The proteasome of the malaria parasite Plasmodium falciparum (Pf20S) is an advantageous drug target because its inhibition kills P. falciparum in multiple stages of its life cycle and synergizes with artemisinins. The 20S proteasome core particle is composed of two antechambers located between an α-ring and a β-ring and a catalytic chamber centrally located between two β-rings. Unfolded peptide substrates must pass through the antechamber before reaching the catalytic chamber for degradation. We recently developed a macrocyclic peptide, TDI-8304, that is highly selective for Pf20S over human proteasomes and is potent in vitro and in vivo against P. falciparum.

To answer this question, we determined a cryo-EM structure of the partially purified β6A117D mutant Pf20S (Pf20Sβ6A117D) with WLW-vs at 2.58 Å resolution. Because WLW-vs is a β2-specific inhibitor, we were surprised to observe WLW-vs in both β2 and β5 catalytic sites of the Pf20Sβ6A117D. The overall binding mode of WLW-vs in both sites is similar, following an anti-parallel β-strand configuration resembling peptide substrates. In both β2 and β5, the inhibitor is covalently linked to the catalytic Thr-1, the two indole groups at the P1 and P3 sites are inserted into the S1 and S3 pockets, respectively, and the P2 Leu and P4 morpholine face the catalytic chamber. We compared the β6 subunit structures of the wild-type Pf20S and A117D mutant Pf20S, and with the high resolution of the two EM maps, we clearly see that the β6A117D caused a one-residue shift as well as an upside-down flip in the Gly156-to-Ala161 region. In the wild-type β6 structure, Tyr158 points upward to interact with the small hydrophobic Ala117. In the A117D mutant β6 structure, the negatively charged Asp117 has expelled Tyr158 from its wild-type position, causing the observed one-residue shift and the upside-down flip in the Gly156-to-Ala161 region. Furthermore, the flipping of the Gly156-to-Ala161 peptide moves Ser154 away from pyrrolidinone and diminishes the TDI-8304’s affinity for the β5 pocket. Also, the aromatic ring of the Tyr158 at its new position hydrophobically interacts with one indole ring of the WLW-vs. Especially, the hydroxyphenyl ring of Tyr158 interacts with the indole ring of the P3 Trp of the WLW-vs via an offset π-π stacking with a favored vertical distance 3.4 Å, which likely explains why the β2-specific inhibitor WLW-vs also binds in the β5 pocket of the Pf20Sβ6A117D, supporting the observed enhanced inhibition against the β5 activity of the Pf20Sβ6A117D19. By comparing the structures of the Pf20S WT and Pf20S A117D, we unambiguously found that the A117D mutation not only causes a conformational change in the β5 inhibitor binding pockets, but also a substantial conformational change remotely in the β2 active subunit that enhances the binding affinity of a β2 inhibitor.

>[2x]MVRPSQSMYDRHLTIFSPDGNLYQIEYAIKAVKNTNITSVGVKGENCAVIISQKKMATQYISQDKLLDYNNITNIYNITDEIGCSMVGMPGDCLSMVYKARSEASEFLYSNGYNVNAETLCRNICDKIQVYTQHAYMRLHACSGMIIGIDENNKPELFKFDPSGFCAGYRACVIGNKEQESISVLERLLEKRKKKIQQETIDEDIRNTTILAIEALQTILAFDLKASEIEVAIVSTKNRNFTQISEKEIDNYLTYIAERD;>MADGEYSFSLTTFSPTGKLVQIEYALNRVSSSSPALGIRAKNGVIIATEKKSPNELIEENSIFKIQQISEHIGIVYAGMPGDFRVLLKRARKEAIRYSLQYGSEILVKELVKIIASIVQEFTQTGGVRPFGLSLLICGVDVYGYHLYQIDPSGCYFNWMATCVGKDYQNNMSFLEKRYNKDIEIEDAIHTAILTLKESYEGVLNEKNIEIGVAYDNKPFKILTQNEIKDYLIEIE[2x];>[2x]MARRYDSRTTTFSPEGRLYQVEYALEAINNASITIGLITKDGVILGADKVFISKLIDKANNYEKIYKIDKHIFCGVAGLNADANILINQSRLYAQRYLYNYNEVQPVSQLVVQICDIKQSYTQYGGLRPYGVSFLIGGYDTKDGYQLYHTDPSGNYSGWFATAIGTNNLTASSVLKQEWKNDMTLEEGLLLALKTLAKSTDTEIPKSEKIELAYLTNKDGEVYQKYLTEKEIEELIKLYTQKYIKE;>MSYDRAITVFSPDGHLLQVEHALEAVKKGGCAVAIKSSNFAVLAVEKKNIPKLQNPKTTEKLIKLDEHNCLAFAGLNADARVLVNKTRLECQRYYLNMDEPAPVDYIAKYVAKVQQKFTHRGGVRPFGIATLIAGFKNNKEICIYQTEPSGIYAAWKAQAIGKNAKIVQEFLEKNYQENMEQKDCIFLALKAIFEVVELSSKNVEVALLTEKDLTFIEEQEINSMVELIDQERTKNNEQNE[2x];>[2x]MFSTRSEYDRGVNTFSPEGRLFQVEYALGAIKLGSTAVGICVNDGVILASERRISSTLIEKDSVEKLLSIDDHIGCAMSGLMADARTLIDYARVECNHYKFIYNENINIKSCVELISELALDFSNLSDSKRKKIMSRPFGVALLIGGVDKNGPCLWYTEPSGTNTRFSAASIGSAQEGAELLLQENYKKDMTFEQAEILALTVLRQVMEDKLSTSNVEICAIKKSDQTFYKYNTDDISRIIDVLPSPVYPTIDMTA;>[2x]MYRNLYDTDNIIYSPEGRLYQVEYASEAIKQGTCAVAIKSKDYVVVSGLKKCISKLSFPQEKIFKIDDYIGISMSGITSDAKVLTKFMQNECLSHKFLYNENINIESLVRSVADKYQKNTQKSSKRAFGVGLMIAAYHNEPCIFETRPNGSYFEYDALSFGARSHASKTYLEKNLHLFEECSLEELILHCLKALKCSLSSESELTISNTALAVVGKNHPWQEISSLQLEEYLSKVKMDAEQEQVEENVQNEANE;>[2x]MAGLSAGYDLSVSTFSPDGRLYQVEYIYKSINNNNTALCLECKDGIICCCINSNMDKNKMIKKNSYNRIYHVNNNIIITYSGFDGDARNIIDRARSEANTYYYNFHTNIPLHILVNRISLYIHAYTLYWHMRPFAASIIISSFNEKDKGDIYCIEPNGACYKYSGIVIGKNKEMFKTEIEKKDYKDINVRDAIEDIYKFILTSDDHMNKNNLQNLVNFSWICKESSYEFQNIHEEILTPALNKAVEYIEKLN;>[2x]TTIIGIIYDNGVMLACDSRTSSGTFISNKCSRKINRINENLYVCRSGASAHSQKIIEIIKHYCVSMKNENRKKGRFHEGETIYDETTYDEEIDIDSINYLDYNNNNDNNLVTKNKYFYEDKFNDYNPLVENVAHITKKIIYTNNNFLSCALIFGGYDKIKKQQLYAVNLNGSIIEKHDFAVSGSGSIYIQSYLQDKYKKFMTKKECFNLILNCVKYAMHNDNSSGGLIRIVNITKSFVEEFTVVNTQMNFQY;>TTICGLVCQNAVILGADTRATEGPIVADKNCSKLHYISKNIWCAGAGVAGDLEHTTLWLQHNVELHRLNTNTQPRVSMCVSRLTQELFKYQGYKVCAIVLGGVDVNGPQLYGIHPHGSSCLLPFTALGSGSLNAMAVLEAKYRDNMTIEEGKNLVCEAICAGIFNDLGSGGNVDICVITKDSYQHIRPYKEPNMRLYHLPHPTIYPKGTTPILSEKIEYIKKFISVEDA[2x];>MGSIYNYNGGCVLGMSGSNCVAIACDLRLGANTFTTVSTKFSKIFKMNNNVYVGLSGLATDIQTLYEILRYRVNLYEVRQDAEMDVECFANMLSSILYSNRFSPYFVNPIVVGFKLKHYVDEEGEKKVNYEPYLTAYDLIGAKCETRDFVVNGVTSEQLFGMCESLYVKDQDENGLFETISQCLLSALDRDCISGWGAEVLVLTPEKIIKKKLKARMD[2x];>[2x]MDTLIGLRGNNFVVLAADTYSINSIIKLKNDDNTKFYDIHGNKCLLLGGSIGDRLQFGEFIRKNVHLYQYQNNTDMFVKSFAFFTRKNLAYYLRRNPFEVNCLIAGYDKKDGYQLYWCDYLSNMDSVNKGAHGYGAYLVSAILDKYYHENLTVDEALDIFKLCFEELKKRFLLTQINYELRIMYDNKVETQYVTV;>[2x]TTTLAFKFKDGIIVAVDSRASMGSFISSQNVEKIIEINKNILGTMAGGAADCLYWEKYLGKIIKIYELRNNEKISVRAASTILSNILYQYKGYGLCCGIILSGYDHTGFNMFYVDDSGKKVEGNLFSCGSGSTYAYSILDSAYDYNLNLDQAVELARNAIYHATFRDGGSGGKVRVFHIHKNGYDKIIEGEDVFDLHYHYTNPEQKDQYVM;>[2x]MDLILYNDNLTEKKTEKENVIEHGRGFKRWYPYIDNGGTVIGLTGKDYVILAADTRLSLSYSIYTRFCPKISKLTDKCIIGSSGMQSDIKTLHSLLQKKIQLFVLEHSHYPDIHVIDRLLCVILYSRRFFPYYAFNILAGVDENNKGVLYNYDSVGSYCEATHSCVGSGSQLILPILDNRVEQKNQLIKNTNFNLGDDINFVKDAITSATERDIYTGDKTLIYVIDKMGINVNTLDLKQD;>MTLGPVVTGTSVIAIKYKHGIMIAADRKASYGSYAKFQNVERIFKINNKTVMGFSGELADAQYLHELLTRKNINNLSEKKRKEDMYTPQHYHSYVSRVFYVRKNRIDPLFNNIIIAGINSQKYDNNDDNVLLYTNKNNDDEQNEYKNNEEYKEIHKDDLYIGFVDMHGTNFCDDYITTGYARYFALTLLRDHYKDNMTEEEARILINECLRILYFRDATSSNFIQIVKVTSKGVEYEEPYILPCVLNSADYVYPSTLLPPAGCMW[2x]4-(1,5-dimethyl-6-oxidanylidene-pyridin-3-yl)benzamide | C14 H14 N2 O2 | 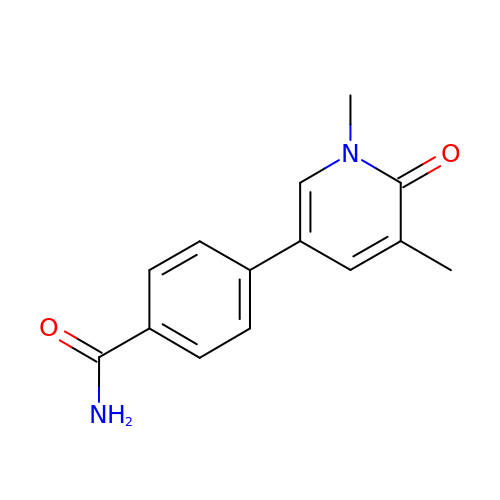LCFYRSDVZKRXGW-UHFFFAOYSA-N> GPLGSPLTASMLASAPPQEQKQMLGE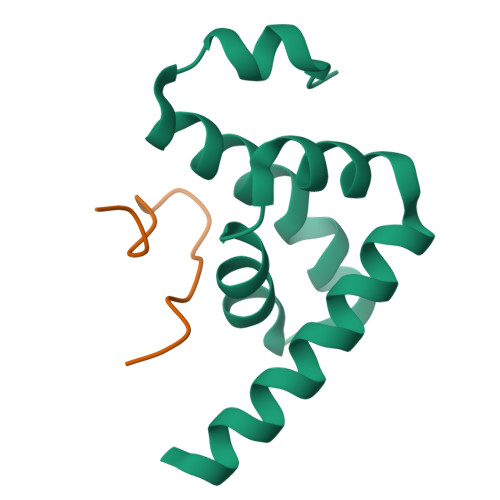RLFPLIQAMHPTLAGKITGMLLEIDNSELLHMLESPESLRSKVDEAVAVLQAHQAKEAAQKA;> GSSINWPPEFHPGVPWKGLQNI> NALPTWWKQAVFYQVYPRSFKDTNGDGIGDLNGIIENLDYLKKLGIDAIWINPHYDSPNTDNGYDIRDYRKIMKEYGTMEDFDRLISEMKKRNMRLMIDIVINHTSDQHAWFVQSKSGKNNPYRDYYFWRDGKDGHAPNNYPSFFGGSAWEKDDKSGQYYLHYFAKQQPDLNWDNPKVRQDLYDMLRFWLDKGVSGLRFATVATYSKIPNFPDLSQQQLKNFAEEYTKGPKIHDYVNEMNREVLSHYDIATAGEIFGVPLDKSIKFFDRRRNELNIAFTFDLIRLDRDADERWRRKDWTLSQFRKIVDKVDQTAGEYGWNAFFLDNHDNPRAVSHFGDDRPQWREHAAKALATLTLTQRATPFIYQGSELGMTNYPFKKIDD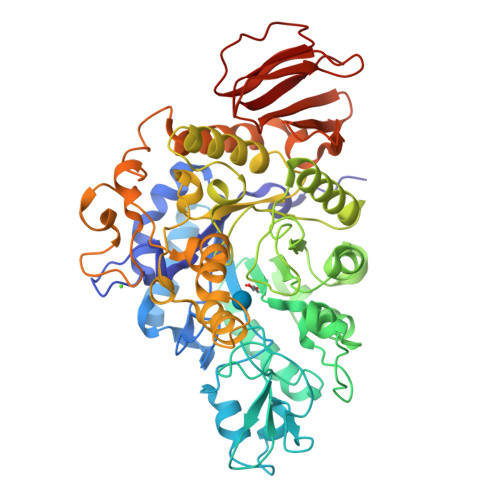FDDVEVKGFWQDYVETGKVKAEEFLQNVRQTSRDNSRTPFQWDASKNAGFTSGTPWLKINPNYKEINSADQINNPNSVFNYYRKLINIRHDIPALTYGSYIDLDPDNNSVYAYTRTLGAEKYLVVINFKEEVMHYTLPGDLSINKVITENNSHTIVNKNDRQLRLEPWQSGIYKLNP> MTYSVSPSSLLTEYGNDNICRVLALDGGGAKGFYTLGVLKEIEAMLGCPLYKRFDLVFGTSTGAIIAALIALGYEVDQIHALYT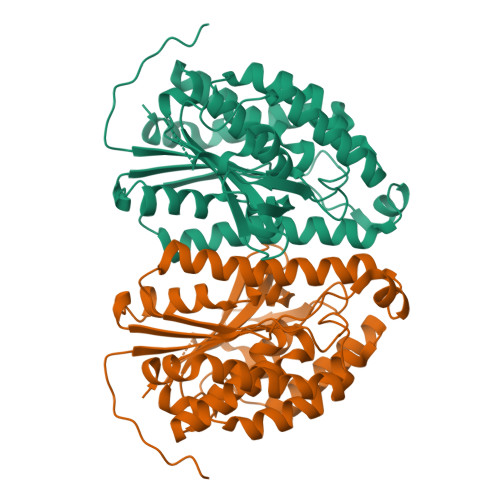EHVPRVMSSRSAAARTMALQDLAKEVFQDKTFEDVLMGIGIVATRWMTERPMIFKGNVVQAHGRKGTFSPGFGVSIADAVQASCSAYPFFERKVIVTAAGDKVELIDGGYCANNPTLFAIADATVALKKDHKDIRVINVGVGIYPEPKPGLLMRIAKKWLAVQLLQKTLEINTQSMDQLRDILFKDIPTIRISDTFERPEMATDLLEYNLDKLNTLRQRGRESFGAREAQLREFLI3-{[(4-{[(2,6-dioxo-1,2,3,6-tetrahydropyrimidin-4-yl)methyl]amino}butyl)amino]methyl}benzoic 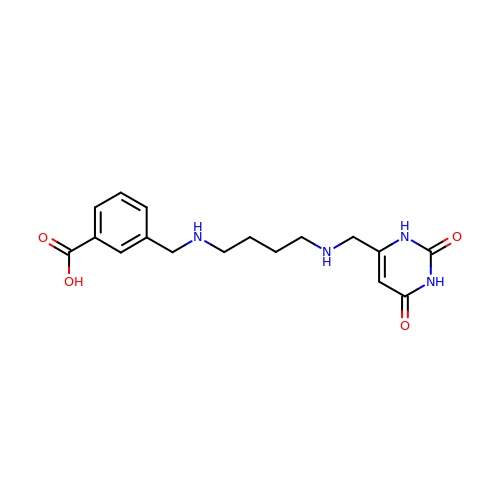acid | C17 H22 N4 O4 | PLKKHOGCWCJFJX-UHFFFAOYSA-N> QTDENRCLKANAKSCGECIQAGPNCGWCTNSTFLQEGMPTSARCDDLEALKKKGCPPDDIENPRGSKDIKKNKNVTNRSKGTAEKLKPEDITQIQPQQLVLRLRSGEPQTFTLKF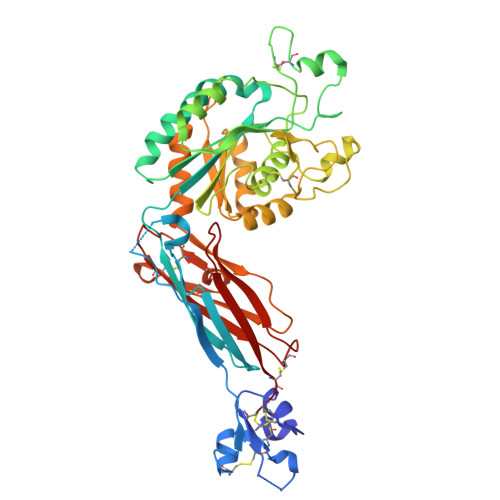KRAEDYPIDLYYLMDLSYSMKDDLENVKSLGTDLMNEMRRITSDFRIGFGSFVEKTVMPYISTTPAKLRNPCTSEQNCTTPFSYKNVLSLTNKGEVFNELVGKQRISGNLDSPEGGFDAIMQVAVCGSLIGWRNVTRLLVFSTDAGFHFAGDGKLGGIVLPNDGQCHLENNMYTMSHYYDYPSIAHLVQKLSENNIQTIFAVTEEFQPVYKELKNLIPKSAVGTLSANSSNVIQLIIDAYNSLSSEVILENGKLSEGVTISYKSYCKNGVNGTGENGRKCSNISIGDEVQFEISITSNKCPKKDSDSFKIRPLGFTEEVEVILQYICECE>[4x]TYCVGIRLDEGLVFASDSRTNAGVDNISTFRKMHVFEVPGERVIVLLTAGNLATTQAVISLLEERLKDPEERLLTAPSMFEAARLVGEALREVQARDAPALEADGVDFNASFILGGQIAGEPPRLFLIYPAGNFIEATPDTPFFQIGETKYGKPILDRVITPDTSLEDAAKCALVSFDSTMRSNLSVGLPLDLLVYERDSLRVGHRRRIDEDDPYFRMLRKQWSEGLRQAFDSLPDPPWE

In 2008, a novel bacterial β subunit homolog, termed Anbu (ancestral β subunit) was identified. We find that Anbu forms a dodecameric open-ring assembly that locally resembles the architecture of the self-compartmentalizing proteasome, but is not closed for steric reasons. The individual subunits are essentially all in the same conformation, assuming the same fold as the proteasomal β subunit. Moreover, a comparison of the active sites shows the catalytic threonine and most other catalytically important residues in essentially the same conformation between Anbu, proteasomal β, and HslV, which suggests the same proteolytic mechanism for all three proteins. Via an extended C-terminal α-helical segment, Anbu forms a dimeric antiparallel coiled-coil interaction across this subunit interface, yielding a 3-fold increased interface area for this dimer compared with the respective subunits in the proteasome.

To test the general validity of our findings, we sought to determine the structure of a second Anbu protein. Therefore, we resorted to a different strategy and designed an Anbu-1 consensus protein (Cons-Anbu), an artificial protein with a sequence corresponding to the most frequently used amino acids in the individual positions of the sequence alignment of all members of the Anbu-1 cluster. Cons-Anbu was indeed highly soluble and even exceeded the thermostability of Pa-Anbu with a Tm of 80°C. Crystallization trials yielded a tetragonal crystal form with two dimers in the asymmetric unit. Around the crystallographic 4-fold screw axis, these two dimers assemble into a helix with eight dimers per turn. The dimers superimpose closely on those of Pa-Anbu with an RMSD of 1.0 Å, and the only noteworthy difference between the two structures lies in the geometry of the helices, which is highly regular in the consensus structure. Also for Cons-Anbu, we did not observe well-defined particles in negative-stain EM, but could visualize elongated helices upon cysteine crosslinking (Cons-AnbuA53CN133C) as for Pa-Anbu.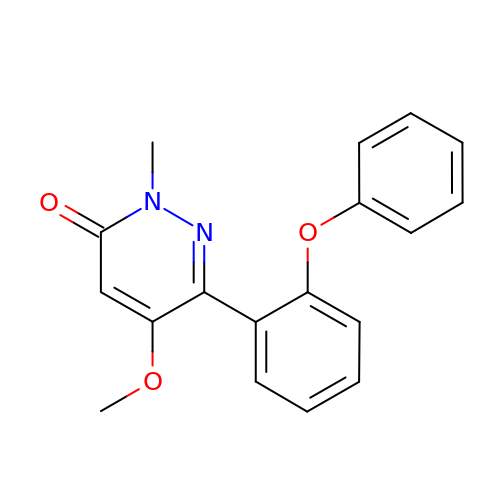5-methoxy-2-methyl-6-(2-phenoxyphenyl)pyridazin-3(2H)-one | C18 H16 N2 O3 | MDTCYTNEBYQKFC-UHFFFAOYSA-N>[2x]MSEKYIVTWDMLQIHARKLASRLMPSEQWKGIIAVSRGGLVPGALLARELGIRHVDTVCISSYDHDNQRELKVLKRAEGDGEGFIVIDDLVDTGGTAVAIREMYPKAHFVTIFAK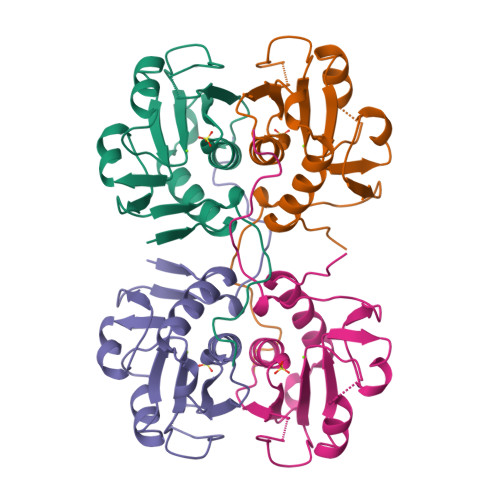PAGRPLVDDYVVDIPQDTWIEQPWDMGVVFVPPISGR>[2x]GSPRTVEEIF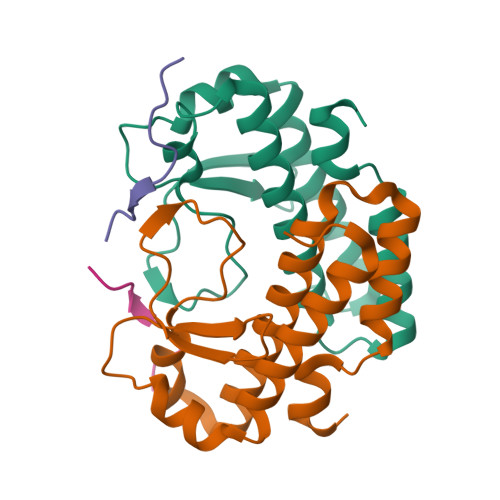KDYSARRAALLRALTKDVDDFYSQCDPEKENLCLYGHPNESWEVNLPAEEVPPELPEPALGINFARDGMQRKDWLSLVAVHSDCWLLSVSFYFGARLNRNERKRLFSLINDLPTLFDVVTGRKAM;>EVRQKKRRKRSTSR[2x]>HPGTHKVYVELQELVMDEKNQELRWMEAARWVQLEENLGENGAWGRPHLSHLTFWSLLELRRVFTKGTVLLDLQETSLAGV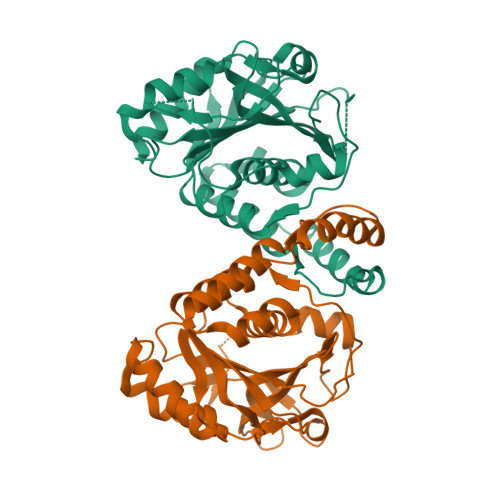ANQLLDRFIFEDQIRPQDREELLRALLLKHSHAGELEALGGVKPAVLTRSGDPSQPLLPQHSSLETQLFCEQGDGGTEGHSPSGILEKIPPDSEATLVLVGRADFLEQPVLGFVRLQEAAELEAVELPVPIRFLFVLLGPEAPHIDYTQLGRAAATLMSERVFRIDAYMAQSRGELLHSLEGFLDCSLVLPPTDAPSEQALLSLVPVQRELLRRRYQSSPAKPDS[2x]>[2x]HHHHHHMRVSFMVAMDENRVIGKDNN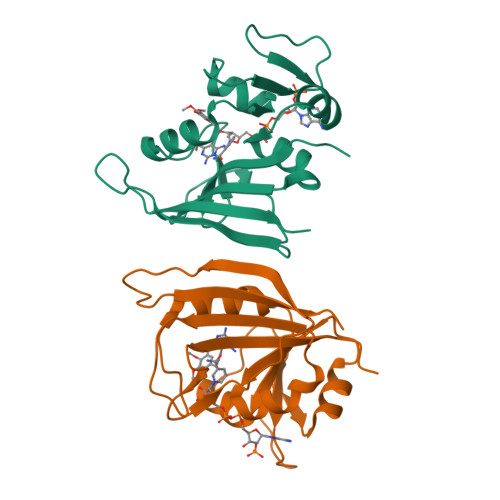LPWRLPSELQYVKKTTMGHPLIMGRKNYEAIGRPLPGRRNIIVTRNEGYHVEGCEVAHSVEEVFELCKNEEEIFIFGGAQIFDLFLPYVDKLYITKIHHAFEGDTFFPEMDMTNWKEVFVEKGLTDEKNPYTYYYHVYEKQQ(1R,3S,5Z)-4-methylidene-5-[(E)-3-[3-[7,7,7-tris(fluoranyl)-6-oxidanyl-6-(trifluoromethyl)hept-3-ynyl]phenyl]pent-2-enylidene]cyclohexane-1,3-diol 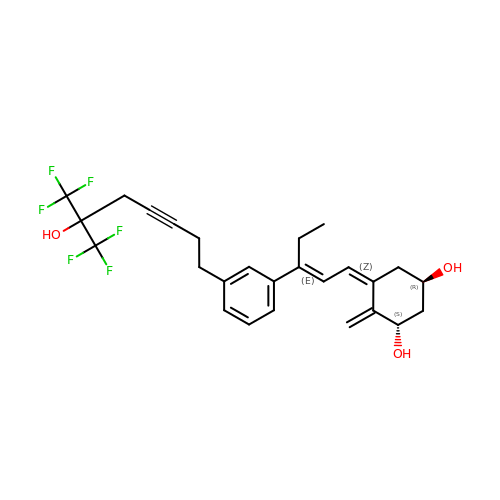| C26 H28 F6 O3 | LEJUFRSKGGKGDS-JRJKOMHBSA-N>[12x]MA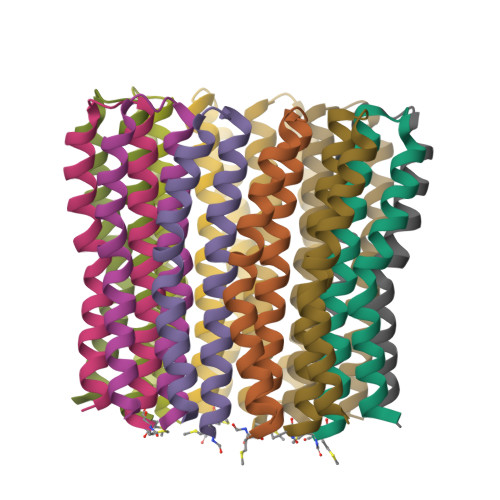FLGAAIAAGLAAVGGAIGVAIIVKATIEGTTRQPELRGTLQTLMFIGVPLAEAVPIIAIVISLLILF>[2x]SDKTFLENNQYTDEGVKVYEFIFGENYISSGGLEATKKILSDIELNENSKVLDIGSGLGGGCMYINEKYGAHTHGIDICSNIVNMANERVSGNNKIIFEANDILTKEFPENNFDLIYSRAAILHLSLENKNKLFQKCYKWLKPTGTLLITDYCATEKENWDDEFKEYVKQRKYTLITVEEYADILTACNFKNVVSKDLSDYWNQLLEVEHKYLHENKEEFLKLFSEKKF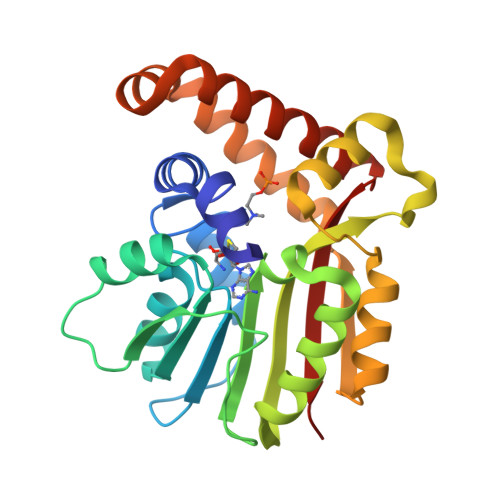ISLDDGWSRKIKDSKRKMQRWGYFKATKN> GGFSWGNYINSNSFIAAPVTCFKHAPMGTCWGDISENVRVEVPNTDCSLPTKVFWIAGIVKLAGYNALLRYEGFENDSGLDFWCNICGSDIHPVGWCAASGKPLVPPRTIQHKYTNWKAFLVKRLTGAKTLPPDFSQKVSESMQYPFKPCMRVEVVDKRHLCRTRVAVVESVIGGRLRLVYEESEDRTDDFWCHMHSPLIHHIGWSRSIGHRFKRSDITKKQDGHFDTPPHLFAKVKEVDQSGEWFKEGMKLEAIDPLNLSTICVATIRKVLADGFLMIGIDGSEAADGSDWFCYHATSPSIFPVGFCEINMIE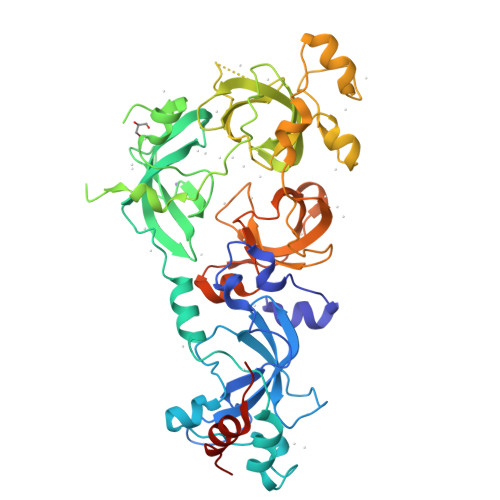LTPPRGYTKLPFKWFDYLRETGSIAAPVKLFNKDVPNHGFRVGMKLEAVDLMEPRLICVATVTRIIHRLLRIHFDGWEEEYDQWVDCESPDLYPVGWCQLTGYQLQPPASGSAGSAGSAGSAGSAGSAQGFVSKTLDSASAQFAASALVTSEQLMG>[6x]ETGHHHHHHDDANVVRDRDLEVDTTLKSLSQQIENIRSPEGSRKNPARTCRDLKMCHSDWKSGEYWIDPNQGCNLDAIKVFCNMETGETCVYPTQPSVAQKNWYISKNPKDKRHVWFGESMTDGFQFEYGGQGSDPADVAIQLTFLRLMSTEASQQ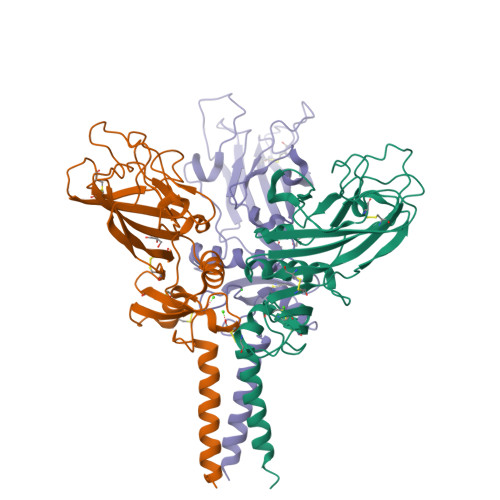ITYHCKNSVAYMDQQTGNLKKALLLQGSNEIEIRAEGNSRFTYSVTVDGCTSHTGAWGKTVIEYKTTKSSRLPIIDVAPLDVGAPDQEFGFDVGPVCFL> MNVRATYTVIFKNASGLPNGYDNWGWGCTLSYYGGAMIINPQEGKYGAVSLKRNSGSFRGGSLRFDMKNEGKVKILVENSEADEKFEVETISPSDEYVTYILDVDFDLPFDRIDFQDAPGNGDRIWIKNLVHSTGSADDFV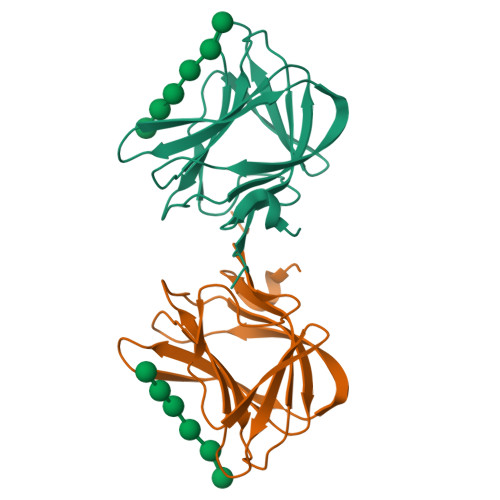DPINLEHHHHHH> MATLSLTVNSGDPPLGALLAVEHVKDDVSISVEEGKENILHVSENVIFTDVNSILRYLARVATTAGLYGSNLMEHTEIDHWLEFSATKLSSSDSFTSTINELNHSLSLRTYLVGNSLSLADLSVWATLKGNAAWQEQLKQKKAPV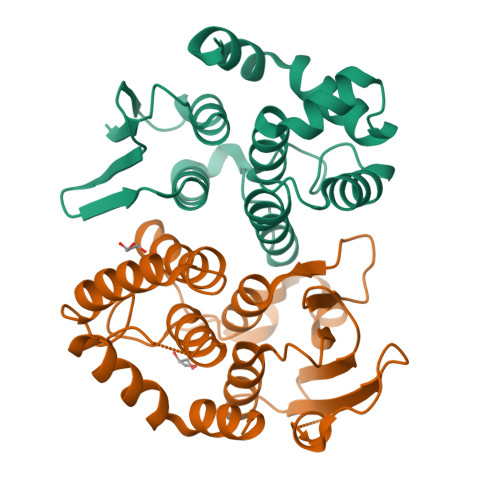HVKRWFGFLEAQQAFQSVGTKWDVSTTKAR;> MTNIIQADEPTTLTTNALDLNSVLGKDYGALKDIVINANPASPPLSLLVLHRLLCEHFRVLSTVHTHDSVKSVPENLLKCFGEQNKKQPRQDYQLGFTLIWKNVPKTQMKFSIQTMCPIEGEGNIARFLFSLFGQKHNAVNATLIDSWVDIAIFQLKEGSSKEKAAVFRSMNSALGKSPWLAGNELTVADVVLWSVLQQIGGCSVTVPANVQRWMRSCENLAPFNTALKLLKLEHHHHHH>[6x]KEMSDRVLIFAVDASGSAAVARLSEAKGAVELLLGRAYAARDHVSLITFRGTAAQVLLQPSRSLTQTKRQLQGLPGGGGTPLASGMEMAMVTAKQARSRGMTPTIALLTDGRGNIALDGTANRELAGEQATKVARAIRASGMPAVIIDTAMRPNPALVDLARTMDAHYIALPRATAHKMADVLGAALEA;>MTTAVARLQPSASGAKTRPVFPFSAIVGQEDMKLALLLTAVDPGIGGVLVFGDRGTGKSTAVRALAALLPEIEAVEGCPVSSPNVEMIPDWATVLSTNVIRKPTPVVDLPLGVSEDRVVGALDIERAISKGEKAFEPGLLARANRGYLYIDECNL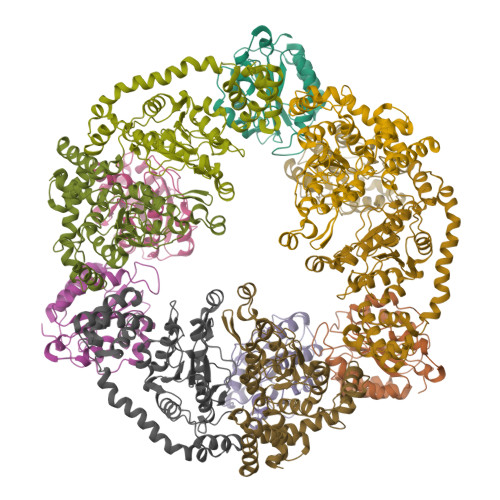LEDHIVDLLLDVAQSGENVVERDGLSIRHPARFVLVGSGNPEEGDLRPQLLDRFGLSVEVLSPRDVETRVEVIRRRDTYDADPKAFLEEWRPKDMDIRNQILEARERLPKVEAPNTALYDCAALCIALGSDGLRGELTLLRSARALAALEGATAVGRDHLKRVATMALSHRLRRDPLDEAGSTARVARTVEETLP[6x]>[4x]MAPVLSKDVADIESILALNPRTQSHAALHSTLAKKLDKKHWKRNPDKNCFHCEKLENNFDDIKHTTLGERGALREAMRCLKCADAPCQKSCPTHLDIKSFITSISNKNYYGAAKMIFSDNPLGLTCGMVCPTSDLCVGGCNLYATEEGSINIGGLQQFASEVFKAMNIPQIRNPCLPSQEKMPEAYSAKIALLGAGPASISCASFLARLGYSDITIFEKQEYVGGLSTSEIPQFRLPYDVVNFEIELMKDLGVKIICGKSLSENEITLNTLKEEGYKAAFIGIGLPEPKTDDIFQGLTQDQGFYTSKDFLPLVAKSSKAGMCACHSPLPSIRGAVIVLGAGDTAFDCATSALRCGARRVFLVFRKGFVNIRAVPEEVELAKEEKCEFLPFLSPRKVIVKGGRIVAVQFVRTEQDETGKWNEDEDQIVHLKADVVISAFGSVLRDPKVKEALSPIKFNRWDLPEVDPETMQTSEPWVFAGGDIVGMANTTVESVNDGKQASWYIHKYIQAQYGASVSAKPELPLFYTPVDLVDISVEMAGLKFINPFGLASAAPTTSSSMIRRAFEAGWGFALTKTFSLDKDIVTNVSPRIVRGTTSGPMYGPGQSSFLNIELISEKTAAYWCQSVTELKADFPDNIVIASIMCSYNKNDWMELSRKAEASGADALELNLSSPHGMGERGMGLACGQDPELVRNICRWVRQAVQIPFFAKLTPNVTDIVSIARAAKEGGADGVTATNTVSGLMGLKADGTPWPAVGAGKRTTYGGVSGTAIRPIALRAVTTIARALPGFPILATGGIDSAESGLQFLHSGASVLQVCSAVQNQDFTVIQDYCTGLKALLYLKSIEELQGWDGQSPGTESHQKGKPVPRIAELMGKKLPNFGPYLEQRKKIIAEEKMRLKEQNAAFPPLERKPFIPKKPIPAIKDV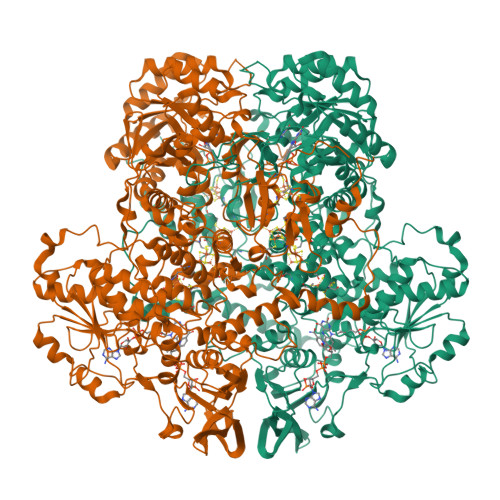IGKALQYLGTFGELSNIEQVVAVIDEEMCINCGKCYMTCNDSGYQAIQFDPETHLPTVTDTCTGCTLCLSVCPIIDCIRMVSRTTPYEPKRGLPLAVNPVC Within each TTSS a conserved, class II chaperone protein is required to prevent premature association of translocator proteins while maintaining them in a secretion competent state, ready to be presented in a temporal fashion to the TTSA. In the enteric pathogen Shigella flexneri, invasion plasmid gene (Ipg) C is the class II chaperone for invasion plasmid antigens (Ipa) B and C. Owing to this central role in supporting translocator function, IpgC is essential for Shigella virulence as an ipgC null strain is noninvasive. Furthermore, upon release of the IpaB and IpaC effectors, IpgC binds to the AraC-like transcription factor, MxiE to promote expression of late-effector genes. Two reports describing high-resolution crystal structures of two class II chaperones have provided a great deal of insight into the structure and function of these all alpha-helical, tetratricopeptide repeat (TPR) proteins.

Here we present the crystal structure of an amino-terminally truncated variant (IpgC10-155) of the Shigella class II secretion chaperone IpgC. In contrast, iterative rounds of likelihood-based molecular replacement using a search model of residues 30-151 of a single IpgC1-151 polypeptide chain eventually provided sufficient information to identify all 18 copies of the IpgC10-155 protein present. Whereas these residues in IpgC1-151 form two short, ordered alpha helices, the same region of IpgC10-155 adopts an extended coil-like structure. However, the dimerization interface of IpgC10-155 observed in our crystal structure is characterized by a rotationally symmetric "head-to-head" arrangement of identical polypeptides chains. The first class of dimer is present in nine crystallographically unique copies and is characterized by a "head-to-head" orientation, where each monomer is related by a single axis of rotational symmetry. This "head-to-head" dimer buries an average of 1262.5 Å2 of surface area upon formation, which compares favorably to the 1381.9 Å2 interface previously described for IpgC1-151. The first of these gives rise to the SycD-like interface (~680 Å2), and involves an intricate array of almost exclusively hydrophobic interactions between the α2 and α3 helices of opposing IpgC10-155 chains. Chief among these is a network of homophilic contacts between Phe residues at positions 46, 58, and 61, whose sidechains nearly intercalate with one another. Separately, a distinct region of contact that masks nearly 580 Å2 of surface area is likewise observed in the IpgC10-155 dimer. This interface arises from packing of nearly the entire extended amino terminus of one IpgC10-155 chain against primarily the α5 helix of its counterpart polypeptide. Comparison of the elution profile of IpgC10-155 to a calibration curve of globular protein standards reveals an observed molecular weight of approximately 36 kDa; given a theoretical value of 16.7 kDa per monomer, this strongly suggests that this amino-terminally truncated IpgC behaves as a dimer in solution.

>[18x]GSTGSSISTAVIDAINSGATLKDINAIPDDMMDDIYSYAYDFYNKGRIEEAEVFFRFLCIYDFYNVDYIMGLAAIYQIKEQFQQAADLYAVAFALGKNDYTPVFHTGQCQLRLKAPLKAKECFELVIQHSNDEKLKIKAQSYLDAIQDIKE>[4x]SMGTK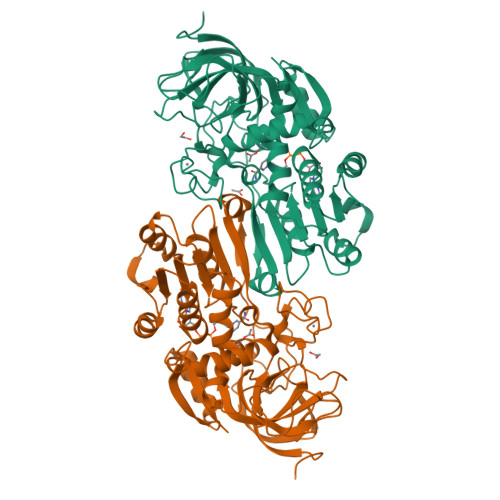GKVIKCKAAIAWEAGKPLCIEEVEVAPPKAHEVRIQIIATSLCHTDATVIDSKFEGLAFPVIVGHEAAGIVESIGPGVTNVKPGDKVIPLYAPLCRKCKFCLSPLTNLCGKISNLKSPASDQQLMEDKTSRFTCKGKPVYHFFGTSTFSQYTVVSDINLAKIDDDANLERVCLLGCGFSTGYGAAINNAKVTPGSTCAVFGLGGVGLSAVMGCKAAGASRIIGIDINSEKFVKAKALGATDCLNPRDLHKPIQEVIIELTKGGVDFALDCAGGSETMKAALDCTTAGWGSCTFIGVAAGSKGLTVFPEELIIGRTINGTFFGGWKSVDSIPKLVTDYKNKKFNLDALVTHTLPFDKISEAFDLMNQGKSIRTILIF> XLGWCIGEAGTD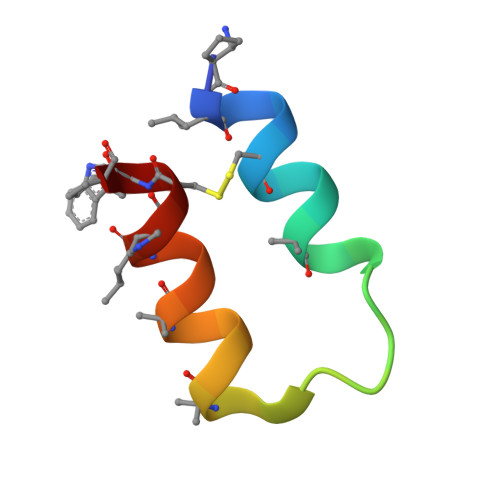PNLNHAQFRAKILXCWX> GSHMDSSISKQALSEIETRHSEIIKLENSIRELHDMFMDMAMLVESQGEMIDRIEYNVEHAVDYVERAVS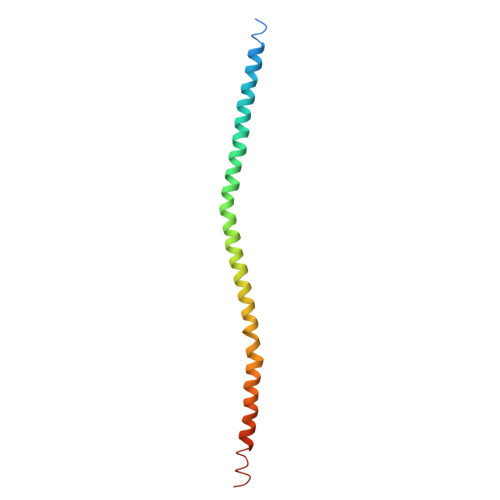DTKKAVKYQSKARRKKIMIIICCVILGIIIASTIGGIFG> Q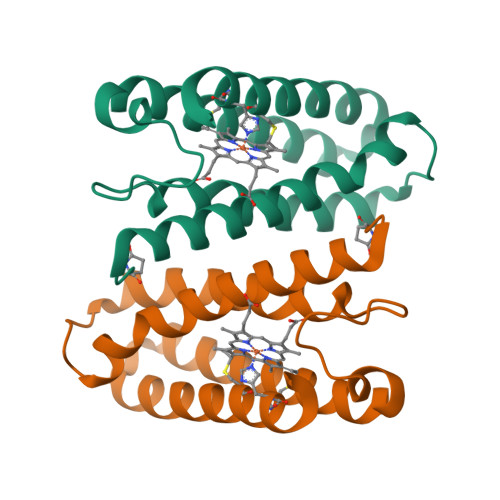FAKPEDAVKYRQSAITLMASHFGRMTPVVKGQAPYDAAQIKANVEVLKTLSALPWAAFGPGTEGGDARPEIWSDAASFKQKQQAFQDNIVKLSAAADAGDLDKLRAAFGDVGASCKACHDAYRK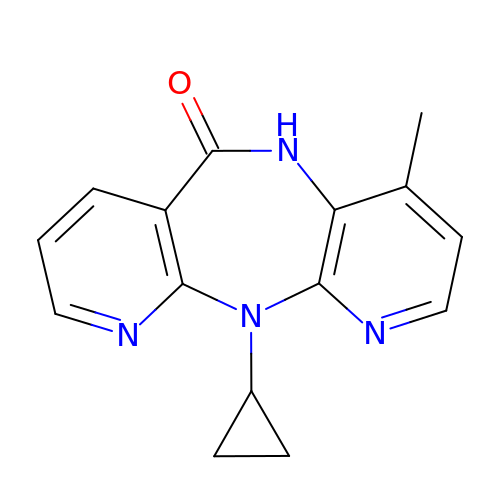11-CYCLOPROPYL-5,11-DIHYDRO-4-METHYL-6H-DIPYRIDO[3,2-B:2',3'-E][1,4]DIAZEPIN-6-ONE | C15 H14 N4 O | NQDJXKOVJZTUJA-UHFFFAOYSA-N> PKFEKNFYQEHPDLARRTAQEVETYRRSKEITVRGHNCPKPVLNFYEANFPANVMDVIARQNFTEPTAIQAQGWPVALSGLDMVGVAQTGSGKTLSYLLPAIVHINHQPFLERGDGPICLVLAPTRELAQQVQQVAAEYCRACRLKSTCIYGGAPKGPQIRDLERGVEICIATPGRLIDFLECGKTNLRRTTYLVLDEADRML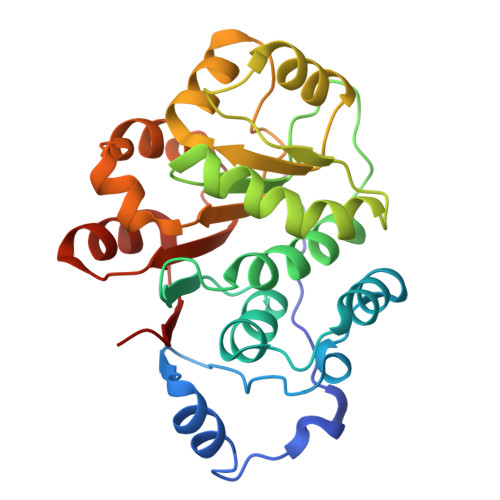DMGFEPQIRKIVDQIRPDRQTLMWSATWPKEVRQLAEDFLKDYIHINIGA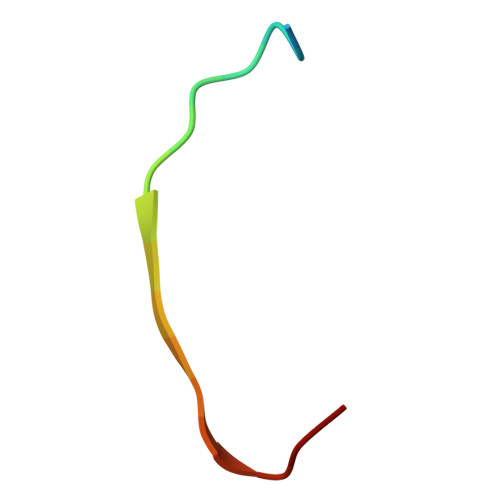> AEQSGKSQTVIVGPWGAQV We also present structures of AvaR1, in isolation (2.4 Å resolution), in complex with avenolide (2.0 Å resolution), and bound to a synthetic DNA oligonucleotide (3.09 Å resolution) derived from its natural binding site. The overall structure is reminiscent of that of other TetR-family transcriptional repressors, and consists of an obligate homodimer. Each monomer is entirely helical and consists of a DNA-binding domain (DBD; composed of α helices 1–4), and a ligand-binding domain (LBD; consisting of α helices 5–13). The dimer interface is formed via interactions between the two LBDs and is formed mainly through hydrophobic packing interactions.

The structure of AvaR1 was determined to 2.4 Å resolution using crystallographic phases determined from anomalous diffraction data collected from SeMet-labeled protein crystals. Notably, the structure of AvaR1 undergoes conformational shifting upon ligand binding, and a structure-based superposition against the ligand-free structure illustrates that binding of the hormone results in an ~10o shift in the DBD of each monomer. This shift results in an increase in the distance between the two DBD in the dimer upon binding of the ligand, which would preclude DNA binding by the ligand-bound homodimer.

>GSENLYFQSGSMARQERAIRTRQTILVAAAEVFDEVGYEAATISDVLKRSGVTKGALYFHFTSKQELAQAVLAEQVASLPRVPEQELKLQQSLDEALLLAHLLREGTGDPIVQGSVRLTVDQGSPRDHLNRRVPMQAWTEHTQSLFEEARAKGEILPHADVEALAKLFVGAFTGVQVLSRIMTGRADLAERVADLYRHLMPSFAMPGILVRLDFSPERGSRVYEAAMKQRESAAASTTDAARTLE[4x]>[2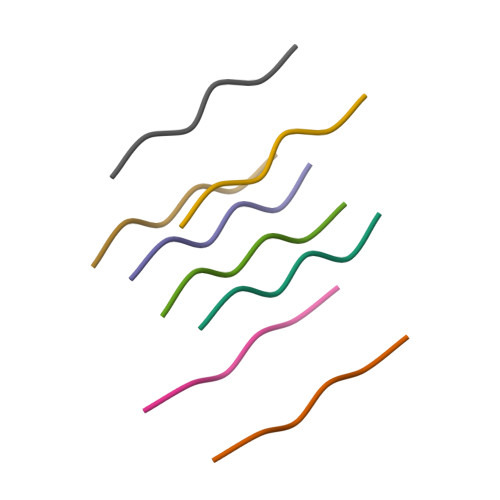x]AEVVFT>[3x]MGSSHHHHHHSQDPMFDIKRKTIEWGGKTLVLETGRIARQADGAVLATMGETVVLATAVFAKSQKPGQDFFPLTVNYQEKTFAAGKIPGGFFKREGRPSEKETLVSRLIDRPIRPLFVKGFKNEVQVVVTVLQHDLENDPDILGMVAASAALCLSGAPFMGPIGAARVGWVDGAYVLNPTLDEMKESKMDLVVAGTADAVMMVESEIQELSEEIVLGGVNFAHQQMQAVIDAIIDLAEHAAKEPFAFEPEDTDAIKAKMKDLVGADIAAAYKIQKKQDRYEAVGAAKKKAIAALGLSDENPTGYDPLKLGAIFKELEADVVRRGILDTGLRIDGRDVKTVRPILGEVGILPRTHGSALFTRGETQAIVVATLGTGDDEQFIDALEGTYKESFLLHYNFPPYSVGETGRMGSPGRREIGHGKLAWRALRPMLPTKEDFPYTIRLVSEITESNGSSSMATVCGSSLAMMDAGVPLVRPVSGIAMGLILEQDGFAVLSDILGDEDHLGDMDFKVAGTSEGLTSLQMDIKIAGITPAIMEQALAQAKEGRAHILGEMNKAMDAPRADVGDFAPKIETINIPTDKIREVIGSGGKVIREIVATTGAKVDINDDGVVKVSASDGAKIKAAIDWIKSITDEAEVGKIYDGKVVKVVDFGAFVNFFGAKDGLVHVSQISNERVAKPSDVLKEGQMVKVKLLGFDDRGKTKLSMKVVDQETGEDLSKKEAAAEEA;>TAPPEKPRRGWWRR[3x]

The phosphorolytic exoribonuclease polynucleotide phosphorylase (PNPase; EC 2.7.7.8) is encoded in the genomes of bacteria and eukaryotes, and in those domains of life the ribonuclease plays multifaceted roles in regulation and environmental response. While the C-terminal RNase PH-like domain catalyses phosphorolytic attack of RNA, the N-terminal domain has lost this capacity; instead, it contributes to the ring-like quaternary structure of the trimeric PNPase assembly. Two recurrent structural motifs that are found in many RNA-binding proteins, the S1 and K-homology (KH) domains, are appended at the C-terminus of PNPase. The PNPase studied here is from the bacterium Caulobacter crescentus, which has been established as a model system to investigate cell cycle progression, because populations can be readily prepared that are synchronized in the cell cycle.

Caulobacter crescentus PNPase was co-crystallized with a short peptide corresponding to its recognition motif from RNase E in two different space groups (P63 and R3). The asymmetric unit of the rhombohedral crystals contains three PNPase protomers, while the hexagonal crystal form contains a single protomer. Although no electron density was apparent for the KH and S1 domains of PNPase in the rhombohedral crystal form, clear density was present for these domains in the hexagonal crystal. Crystals of RNA-free PNPase with recognition peptide (KPRRGWWR) revealed clear density for the peptide in both the hexagonal and rhombohedral crystal forms of PNPase. For the rhombohedral crystal form, eight residues of the peptide could be modelled into this density. The GWW motif occupies a hydrophobic pocket formed by the loop connecting helix α2 and strand β7, and the linker region between helices α5 and α6 on the surface of PNPase (figure 4a(i)). The interaction between PNPase and the RNase E recognition motif in C. crescentus is markedly different from that seen in E. coli. In our C. crescentus structure, it is clear that the GWW motif is buried into a hydrophobic pocket on the surface of PNPase, at a site approximately 60 Å from the position corresponding to the RNase E recognition site in E. coli. This is a fascinating example of convergent evolution, where different bacterial classes have arrived at distinct means of recruiting PNPase into a complex with RNase E.>[8x]PKLV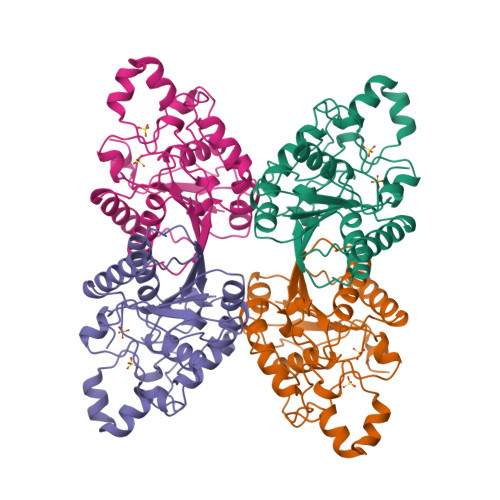LVRHGQSEWNEKNLFTGWVDVKLSAKGQQEAARAGELLKEKKVYPDVLYTSKLSRAIQTANIALEKADRLWIPVNRSWRLNERHYGDLQGKDKAETLKKFGEEKFNTYRRSFDVPPPPIDASSPFSQKGDERYKYVDPNVLPETESLALVIDRLLPYWQDVIAKDLLSGKTVMIAAHGNSLRGLVKHLEGISDADIAKLNIPTGIPLVFELDENLKPSKPSYYLDPEAAAAGAAAVANQGKK>MERAESSSTEPAKAIKPIDRKSVHQICSGQVVLSLSTAVKELVENSLDAGATNIDLKLKDYGVDLIEVSDNGCGVEEENFEGLTLKHHTSKIQEFADLTQVETFGFRGEALSSLCALSDVTISTCHASAKVGTRLMFDHNGKIIQKTPYPRPRGTTVSVQQLFSTLPVRHKEFQRNIKKEYAKMVQVLHAYCIISAGIRVSCTNQLGQGKRQPVVCTGGSPSIKENIGSVFGQKQLQSLIPFVQLPPSDSVCEEYGLSCSDALHNLFYISGFISQCTH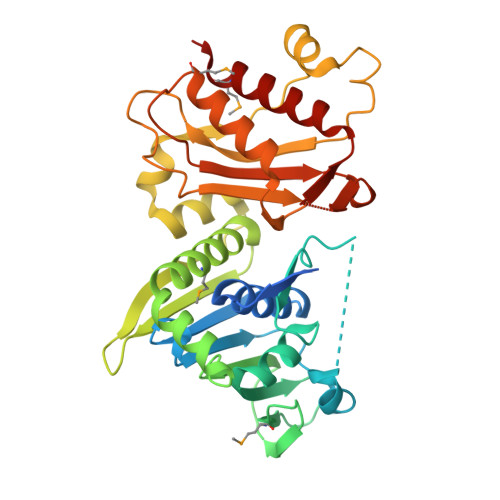GVGRSSTDRQFFFINRRPCDPAKVCRLVNEVYHMYNRHQYPFVVLNISVDSECVDINVTPDKRQILLQEEKLLLAVLKTSLIGMFDS[2x]> GAASMEFPFDVDALFPERITVLDQHLRPPARRPGTTTPARVDLQQQIMTIIDELGKASAKAQNLSAPITSASRMQSNRHVVYILKDSSARPAGKGAIIGFIKVGYKK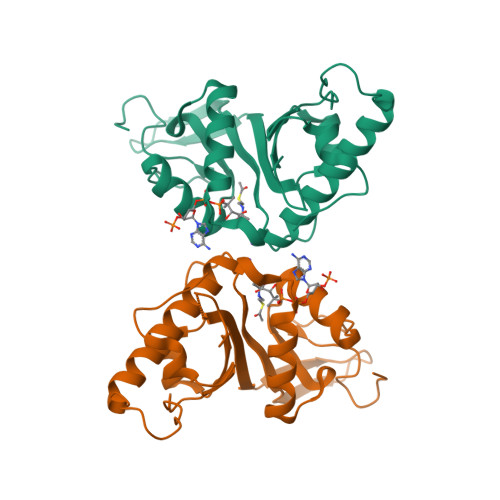LFVLDDREAHNEVEPLCILDFYIHESVQRHGHGRELFQYMLQKERVEPHQLAIDRPSQKLLKFLNKHYNLETTVPQVNNFVIFEGFFAHQHRP> QLTPTFYDNSCPNVSNIVRDTIVNELRSDPRIAASILRLHFHDCFVNGCDASILLDNTTSFRTEKDAFGNANSARGFPVIDRMKAAVESACPRTVSCADLLTIAAQQSVTLAGGPSWRVPLGRRDSLQAFLDLANANLPAPFFTLPQLK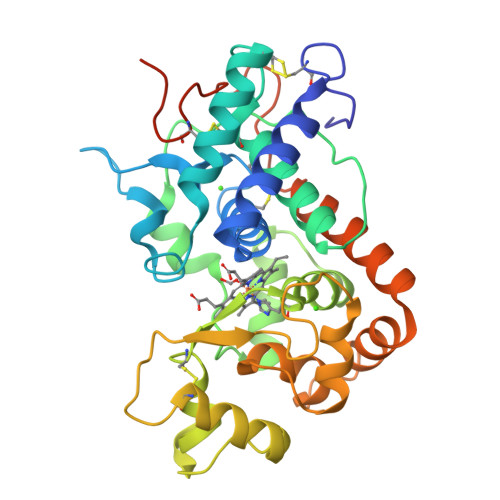DSFRNVGLNRSSDLVALSGGHTFGKNQCRFIMDRLYNFSNTGLPDPTLNTTYLQTLRGLCPLNGNLSALVDFDLRTPTIFDNKYYVNLEEQKGLIQSDQELFSSPNATDTIPLVRSFANSTQTFFNAFVEAMDRMGNITPLTGTQGQIRLNCRVVNSNSLLHDMVEVVDFVSSM>[6x]SVSDTNLYSPFKPRNYQLELALPAMKGKNTIICAPTGCGKTFVSLLICEHHLKKFPQGQKGKVVFFANQIPVYEQQKSVFSKYFERHGYRVTGISGATAENVPVEQIVENNDIIILTPQILVNNLKKGTIPSLSIFTLMIFDECHNTSKQHPYNMIMFNY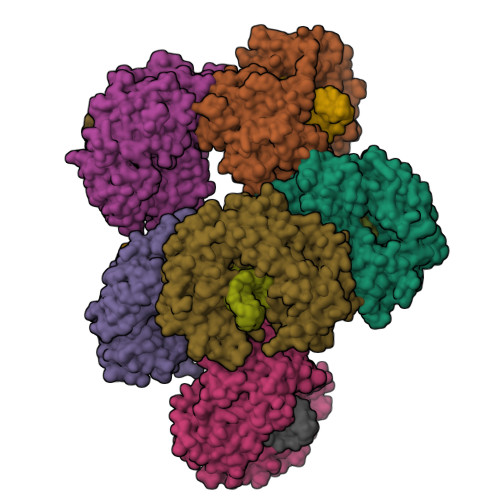LDQKLGGSSGPLPQVIGLTASVGVGDAKNTDEALDYICKLCASLDASVIATVKHNLEELEQVVYKPQKFFRKVESRISDKFKYIIAQLMRDTESLAKRICKDLENLSQIQNREFGTQKYEQWIVTVQKACMVFQMPDKDEESRICKALFLYTSHLRKYNDALIISEHARMKDALDYLKDFFSNVRAAGFDEIEQDLTQRFEEKLQELESVSRDPSNENPKLEDLCFILQEEYHLNPETITILFVKTRALVDALKNWIEGNPKLSFLKPGILTGRGKTNQNTGMTLPAQKCILDAFKASGDHNILIATSVADEGIDIAQCNLVILYEYVGNVIKMIQTRGRGRARGSKCFLLTSNAGVIEKEQINMYKEKMMNDSILRLQTWDEAVFREKILHIQTHEKFIRDSQEKPKPVPDKENKKLLCRKCKALACYTADVRVIEECHYTVLGDAFKECFVSRPHPKPKQFSSFEKRAKIFCARQNCSHDWGIHVKYKTFEIPVIKIESFVVEDIATGVQTLYSKWKDFHFEKIPFDPAEMSK N-methyl-N'-(3-methylbut-2-en-1-yl)-N'-(3-phenoxyphenyl)-N-[trans-4-(pyridin-4-yl)cyclohexyl]urea 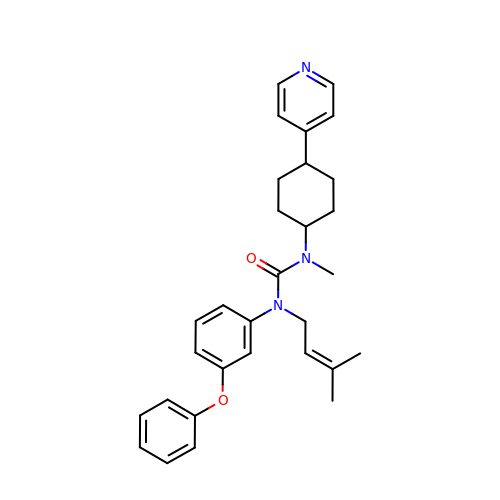| C30 H35 N3 O2 | ZAXRBGRMBUAKGI-YOCNBXQISA-N> GASPSAQELKEQGNRLFVGRKYPEAAAC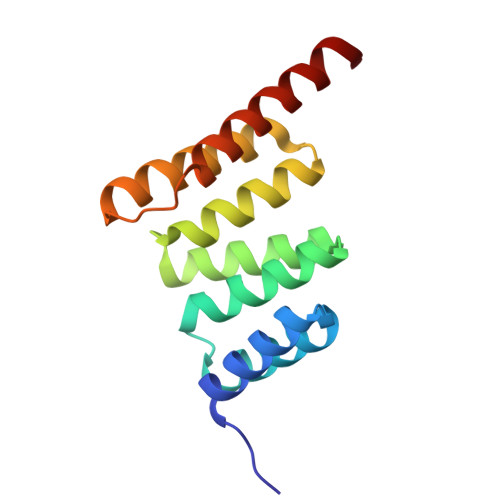YGRAITRNPLVAVYYTNRALCYLKMQQHEQALADCRRALELDGQSVKAHFFLGQCQLEMESYDEAIANLQRAYSLAKEQRLNFGDDIPSALRIAKKKRWNSIEERR2-[(1R,2R,5S)-5-methyl-2-(prop-1-en-2-yl)cyclohexyl]-5-pentylbenzene-1,3-diol | C21 H32 O2 | 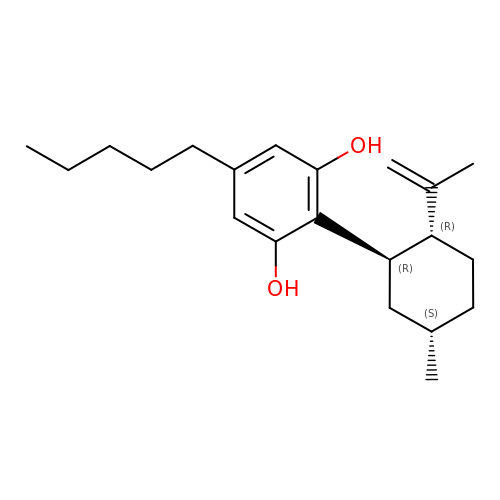CODIXLGYYWMJFS-RYQLBKOJSA-N> MRAEGLGGLERFCSPGKGRGLRALQPFQVGDLLFSCPAYAYVLTVNERGNHCEYCFTRKEGLSKCGRCKQAFYCNVECQKEDWPMHKLECSPMVVFGENWNPSETVR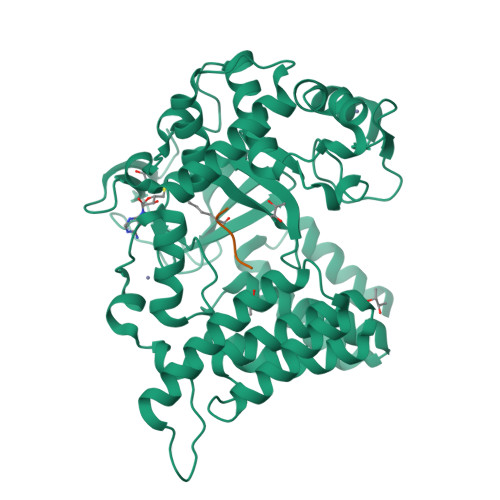LTARILAKQKIHPERTPSEKLLAVKEFESHLDKLDNEKKDLIQSDIAALHHFYSKHLEFPDNDSLVVLFAQVNCNGFTIEDEELSHLGSAIFPDVALMNHSCCPNVIVTYKGTLAEVRAVQEIKPGEEVFTSYIDLLYPTEDRNDRLRDSYFFTCECQECTTKDKDKAKVEIRKLSDPPKAEAIRDMVRYARNVIEEFRRAKHYKSPSELLEICELSQEKMSSVFEDSNVYMLHMMYQAMGVCLYMQDWEGALQYGQKIIKPYSKHYPLYSLNVASMWLKLGRLYMGLEHKAAGEKALKKAIAIMEVAHGKDHPYISEIKQEIESH;> SSHLKSKKGQSTS>MAEELVLERCDLELETNGRDHHTADLCREKLVVRRGQPFWLTLHFEGRNYEASVDSLTFSVVTGPAPSQEAGTKARFPLRDAVEEGDWTATVVDQQDCTLSLQLTTPANAPIGLYRLSLEASTGYQGSSFVLGHFILLFNAWCPADAVYLDSEEERQEYVLTQQGFIYQGSAKFIKNIPWNFGQFEDGILDICLILLDVNPKFLKNAGRDCSRRSSPVYVGRVVSGMVNCNDDQGVLLGRWDNNYGDGVSP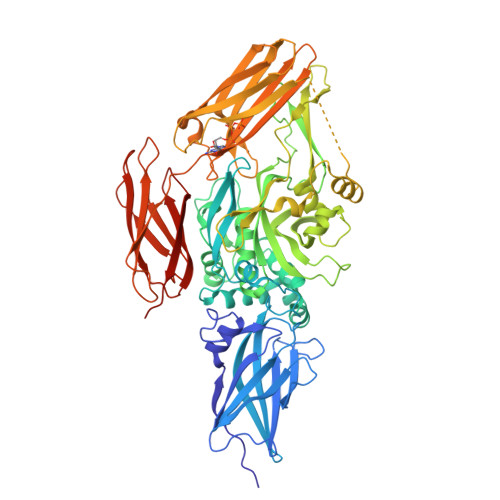MSWIGSVDILRRWKNHGCQRVKYGQCWVFAAVACTVLRCLGIPTRVVTNYNSAHDQNSNLLIEYFRNEFGEIQGDKSEMIWNFHCWVESWMTRPDLQPGYEGWQALDPTPQEKSEGTYCCGPVPVRAIKEGDLSTKYDAPFVFAEVNADVVDWIQQDDGSVHKSINRSLIVGLKISTKSVGRDEREDITHTYKYPEGSSEEREAFTRANHLNKLAEKEETGMAMRIRVGQSMNMGSDFDVFAHITNNTAEEYVCRLLLCARTVSYNGILGPECGTKYLLNLNLEPFSEKSVPLCILYEKYRDCLTESNLIKVRALLVEPVINSYLLAERDLYLENPEIKIRILGEPKQKRKLVAEVSLQNPLPVALEGCTFTVEGAGLTEEQKTVEIPDPVEAGEEVKVRMDLLPLHMGLHKLVVNFESDKLKAVKGFRNVIIGPALEHHHHHH[3x]> SNAMETFLFTSESVNEGHPDKLCDQISDAVLDACLEQDPDSKVACETCTKTNMVMVFGEITTKATVDYEKIVRDTCRAIGFVSDDVGLDADKCKVLVNIEQQSPDIAQGVHGHFTKCPEEIGAGDQGHMFGYATDETPELMP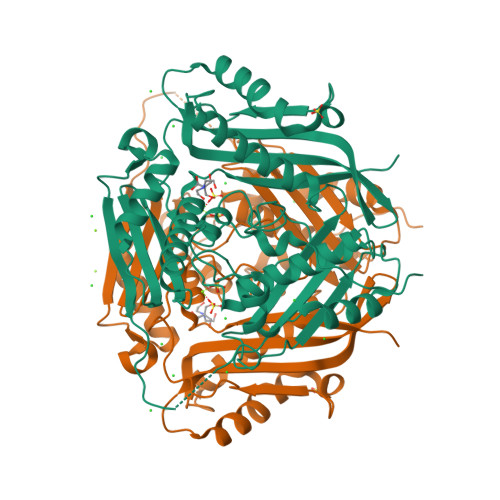LSHVLATKLGARLTEVRKNGTCAWLRPDGKTQVTVEYYNDKGAMVPIRVHTVLISTQHDETVTNDEIARDLKEHVIKPVIPEKYLDEKTIFHLNPSGRFVIGGPHGDAGLTGRKIIIDTYGGWGAHGGGAFSGKDPTKVDRSGAYIVRQAAKSVVANGMARRALVQVSYAIGVPEPLSVFVDTYETGLIPDKEILKIVKESFDFRPGMMTINLDLKRGGNGRFLKTAAYGHFGRDDPDFTWEVVKPLKWDKPQA>[2x]GIDPFTMTPSEDFVVTDRGGIVENSHRVHAAVVDAKGRLLYALGNPTRMTLARSAAKPAQALAILETEGVAGY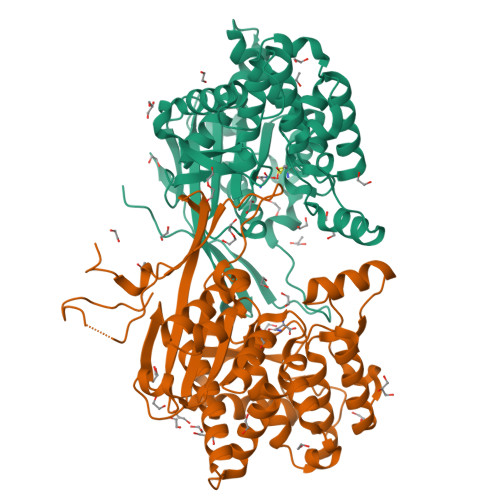GFDDADIALMCASHSSEDRHIARTRAMLSKIKAEEADLRCGGHPSLSEMVNRSWIKQDFIPTAVCSNCSGAHVGMLAGARAIGAGTDGYHLPDHPMQGRVKRTVAELCDLDAGDVEWGTDGCNLPTPAFPLDRLGRIYAKLASAADGSDAGEGQSTRCAALAHIFRAMARHPEMVAGEGRYCTMLMRAFDGALVGKLGADASYAIGVRASDATRQLGTDGALGISVKIEDGNLEMLYAVVTELLERLGIGSPDVRSQLASFHHPQRVNTMGVTTGGVSFPFKLRGSKSNVDDPRLAAVAR>VAEKAKDERELLEKTSELIAGMGDKIGEHLGDKYKAIAKDIADNIKNFQGKTIRSFDDAMASLNKITANPAMKINKADRDALVNAWKHVDAQDMANKLGNLS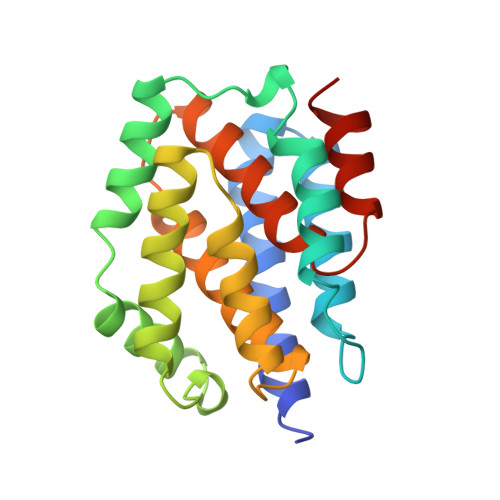KAFKVADVVMKVEKVREKSIEGYETGNWGPLMLEVESWVLSGIASSVALGIFSATLGAYALSLGVPAIAVGIAGILLAAVVGALIDDKFADALNNEIIRPAH[2x]> IETVPVKLKPGMDGPKVKQWPLTEEKIK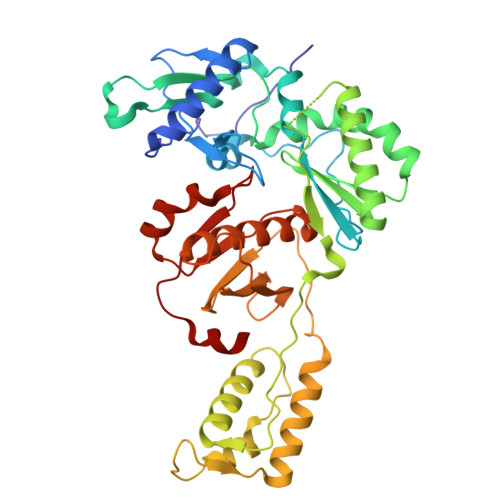ALVEICTEMEKEGKISKIGPENPYNTPVFAIKKKDSTKWRKLVDFRELNKRTQDFWEVQLGIPHPAGLKKKKSVTVLDVGDAYFSVPLDEDFRKYTAFTIPSINNETPGIRYQYNVLPQGWKGSPAIFQSSMTKILEPFKKQNPDIVIYQYMDDLYVGSDLEIGQHRTKIEELRQHLLRWGLFLWMGYELHPDKWTVQPIVLPEKDSWTVNDIQKLVGKLNWASQIYPGIKVRQLSKLLRGTKALTEVIPLTEEAELELAENREILKEPVHGVYYDPSKDLIAEIQKQGQGQWTYQIYQEPFKNLKTGKYARMRGAHTNDVKQLTEAVQKITTESIVIWGKTPKFKLPIQKETWETWWTEYWQATWIPEWEFVNTPPLVKLWYQ> SMPPKASKKDAAPAERPILGRFSSHLKIGIVGLPNVGKSTFFNIVTKLSIPAENF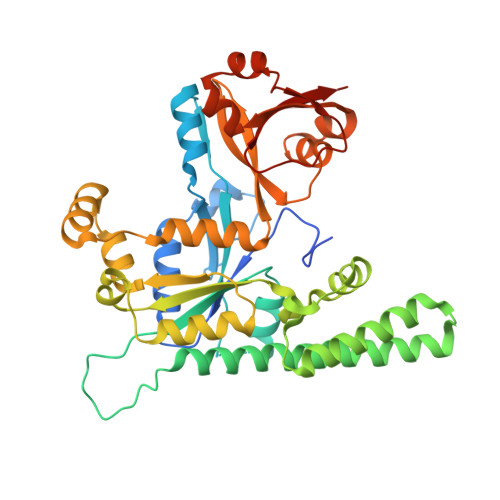PFCTIDPNEARVYVPDERFDWLCQLYKPKSEVSAYLEINDIAGLVRGAHAGEGLGNAFLSHIRAVDGIFHVLRAFEDKEVTHIDDSVDPVRDLETIGEELRLKDIEFVQNKIDDLEKSMKRSNDKQLKLEHELCEKVKAHLEDGKDVRFGDWKSADIEILNTFQLLTAKPVVYLVNMSEKDYQRKKNKFLPKIHAWVQEHGGETIIPFSCAFERLLADMPPDEAAKYCAENQIASVIPKIIKTGFAAIHLIYFFTAGPDEVKCWQIRRQTKAPQAAGTIHTDFERGFICAEVMKFDDLKELGSESAVKAAGKYRQEGKTYVVQDGDIIFFKFNVSGGGKK> GSHMASMAKTLKDLQGWEIITTDEQGNIIDGGQKRLRRRGAKTEHYLKRSSDGIKLGRGDSVVMHNEAAGTYSVYMIQELRLNTLNNVVELWALTYLRWFEVNPLAHYRQFNPDANILNRPLNYYNKLFSETANKNELYLTAELAELQLFNFIRVANVMDGSKWEVLKGNVDPERDFTVRYICEPTGEKFVDINIEDVKAYIKKVEPREAQEYLKDLTLPSKKKE;> GSHMASEKKFSTEEEYVSPRFLVADGFLIDLAEEK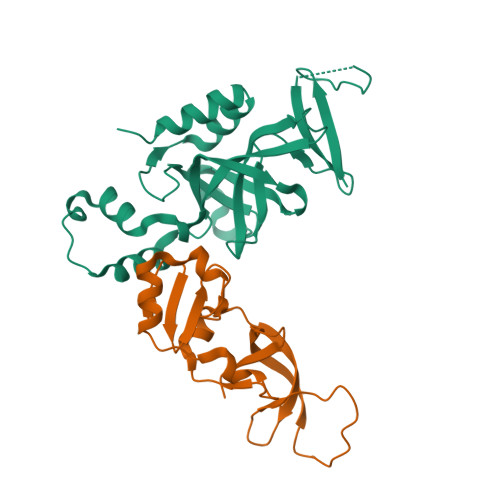PINPKDPRLLTLLKDHQRAMIDQMNLVKWNDFKKYQDPIPLKAKTLFKFCKQIKKKFLRGADFKLHTLPTEANLKYEPERMTVLASCVPILLDDQTVQYLYDD>[4x]SMRKSREYEHVRRDLDPNEVWEIVGELGDGAFGKVYKAKNKETGALAAAKVIETKSEEELEDYIVE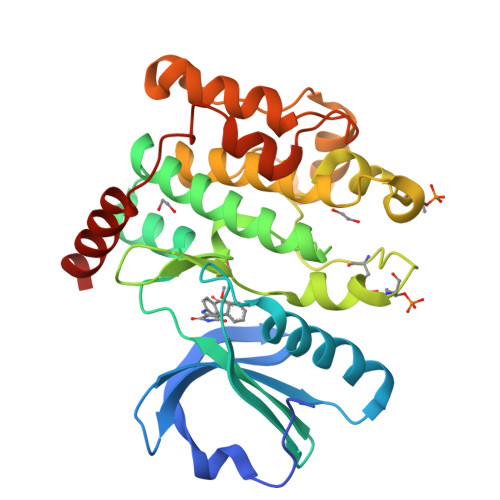IEILATCDHPYIVKLLGAYYHDGKLWIMIEFCPGGAVDAIMLELDRGLTEPQIQVVCRQMLEALNFLHSKRIIHRDLKAGNVLMTLEGDIRLADFGVSAKNLKTLQKRDSFIGTPYWMAPEVVMCETMKDTPYDYKADIWSLGITLIEMAQIEPPHHELNPMRVLLKIAKSDPPTLLTPSKWSVEFRDFLKIALDKNPETRPSAAQLLEHPFVSSITSNKALRELVAEAKAEVMEE>GPVPYRQIDDCPAKARPQHIFYRRFLGKDGRRDPKCQWKFAVIFWGNDPYGLKKLSQAFQFGGVKAGPVSCLPHPGP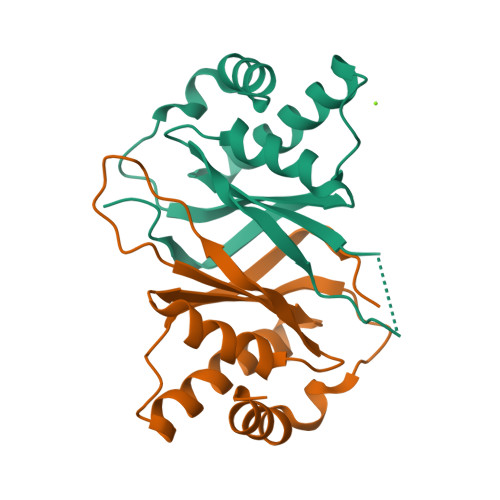DQSPITYCVYVYCQNKDTSKKVQMARLAWEASHPLAGNLQSSIVKFKKPLPLTQPGE[8x]>[8x]ARQERAAQTRRTIVAAAAAVFDELGYEATTIAEILKRSGVTKGALYFHFTSKEQLAQEVLTSQLRAVPPVEEQRLVLQQIIDETLLLAQLLSKGDPLVRGSVRLTVEPG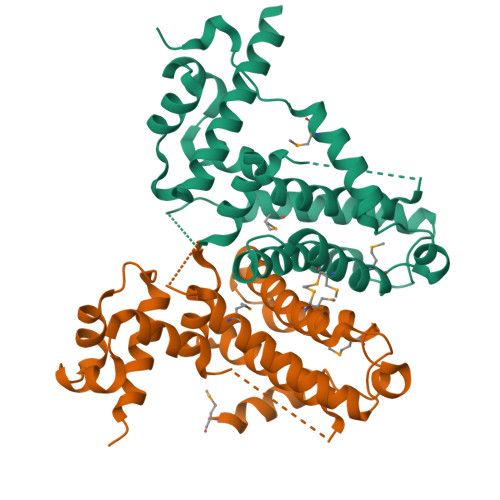APRDGLDRRAPMQEWIGHGRDLLRRAEAGGELLPRLDVDAVARMLVGGFTGAQILSNILTGHADLLERVTDMHRHLMTSVAVPAVLVRLDFSAERSITVYDEAMRRREAPLPAAGDLEH>SFFSFLGEAFDGARDMWRAYSDMREANYIGSDKYFHARGNYDAAKRGPGGVWAAEAISDARENIQR[12x]

The disease arises in mice and humans from the misfolding of the acute phase protein serum amyloid A1 (SAA1). To investigate the molecular basis of the systemic AA amyloidosis, we here use electron cryo-microscopy (cryo-EM) and determined the structures of AA amyloid fibrils from a patient and from a diseased mouse. The human fibril encloses a clearly discernible cavity that contains many charged and polar amino acid residues, making it likely that the vacant space in the cavity is filled with water. Both fibril proteins adopt all-beta folds and differ sharply from the known globular conformations of SAA family members. The murine and the human fibril possess in-register, parallel cross-β sheets and adopt highly similar β-arch conformations at the protein N-termini.

The human fibril proteins originate from human hSAA1.1 and mainly represent the fragments hSAA1.1(2–64) and hSAA1.1(2–47). The ordered part of the density of the mouse fibril corresponds to residues 1–69 of mSAA1.1, the ordered part of the human fibril to hSAA1.1 residues 2–55. The dominant human morphology is 8.1 ± 0.5 nm wide and possesses a cross-over distance of 55.2 ± 1.7 nm (measurements were obtained from cryo-EM images). By contrast, platinum side shadowing demonstrates that the human fibril is right-hand twisted and contains right-hand twisted β-sheets. The human fibril protein contains no amyloid key fold. The human fibril exhibits a considerably larger interface containing polar, ionic, and hydrophobic cross-stack interactions. The center of the human fibril is formed by a steric zipper, which shows a self-complementary packing of the sheets β3 from the two protein stacks. Our reconstruction shows that the N-terminus of the human protein, which lacks the N-terminal Arg, is located within the tightly packed fibril core. The N-terminal α-amino groups form salt bridges to the β-carboxyl groups of Asp33.> MNSDEVQLIKKTWEIPVATPTDSGAAILTQFFNRFPSNLEKFPFRDVPLEELSGNA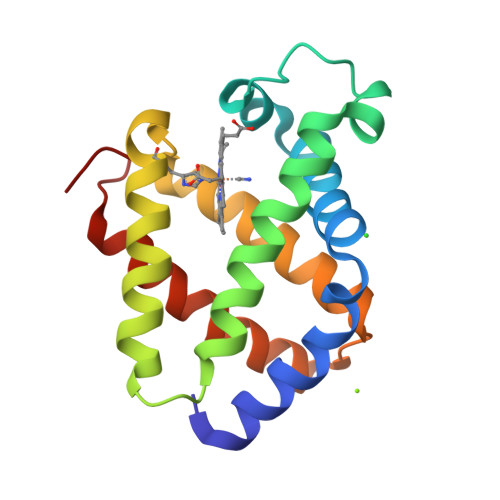RFRAHAGRIIRVFDESIQVLGQDGDLEKLDEIWTKIAVSHIPRTVSKESYNQLKGVILDVLTAASSLDESQAATWAKLVDHVYGIIFKAIDDDGNAK> MDEAVGDLKQALPCVAESPTVHVEVHQRGSSTAKKEDINLSVRKLLNRHNIVFGDYTWTEFDEPFLTRNVQSVSIIDTELKVKDSQPIDLSACTVALHIFQLNEDGPSSENLEEETENIIAANHWVLPAAEFHGLWDSLVYDVEVKSHLLDYVMTTLLFS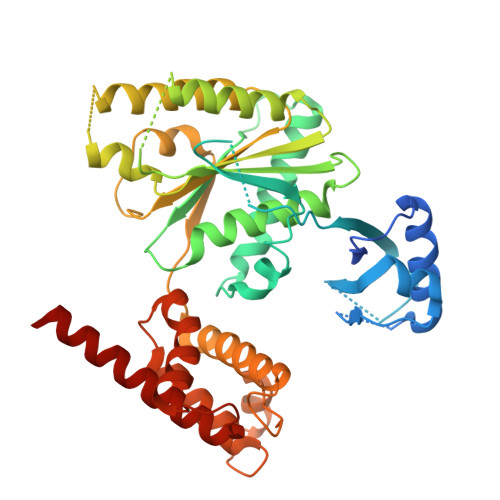DKNVNSNLITWNRVVLLHGPPGTGKTSLCKALAQKLTIRLSSRYRYGQLIEINSHSLFSKWFSESGKLVTKMFQKIQDLIDDKDALVFVLIDQVESLTAARNACRAGTEPSDAIRVVNAVLTQIDQIKRHSNVVILTTSNITEKIDVAFVDRADIKQYIGPPSAAAIFKIYLSCLEELMKCQIIYPRQQLLTLRELEMIGFIENNVSKLSLLLNDISRKSEGLSGRVLRKLPFLAHALYVQAPTVTIEGFLQALSLAVDKQFEERKKLAAYI> DAASDLKSRLDKV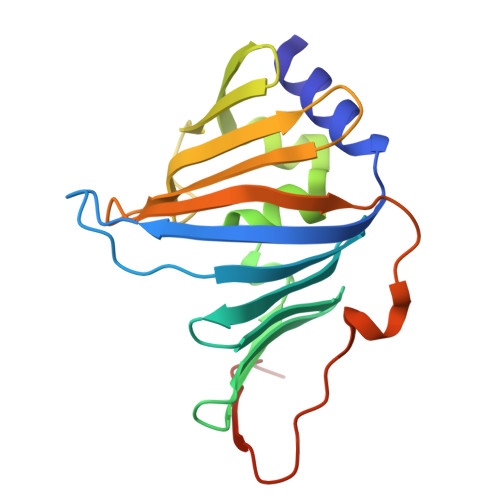SSFHASFTQKVTDGSGAAVQEGQGDLWVKLPNLFNWHMTQPDESILVSDGKTLWFYNPFVEQATATWLKDATGNTPFMLIARNQSSDWQQYNIKQNGDDFVLTPKASNGNLKQFTINVGRDGTIHQFSAVEQDDQRSSYQLKSQQNGAVDAAKFTFTPPQGVTVDDQRKLEHHHHHH> MTLYMGPNTGLLINGLPGEGHYSDLIRMWRWDDFLRQPVVKGRVATLPTTGQAEGDTYIFTGSGSNQNRLARWWATGATTAIWEYMPPRLGWRVQVANETTPSGQVKTYEYSGTAWVELVGGMS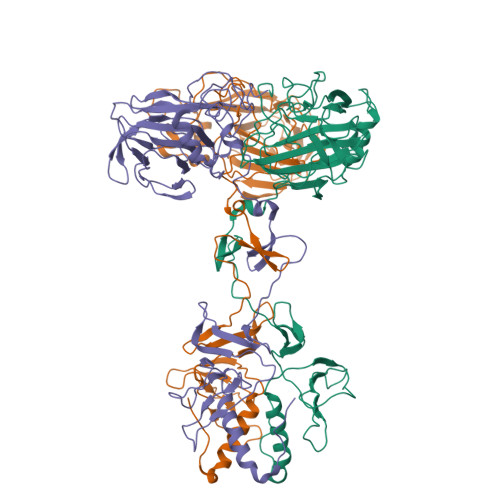DAPSDGKAYARESGAWTELGSAAKSALNVLPFMNLMPDMGRFAGTAANPLATMFTTSWTPSSFLNGWNGATVADGGKFAFDNSTNGGAGPALNARVQALLAAMGRTWTSVSRYGVEFFTAVLTAGSQTTTGSAGADGVTRYLCCSNGSKTVFNAGGWATVVMWLRVESGSAHISSAPYTTHRLWINGAVAAPGVVLPANQWVHLRFSMQSYNGYDNACPYIYASAGAQIAFACPAWFGGLVDPGIHVAPILTINGASA> MKLSRISAINWNKIQDDKDLEVWNRLTSNFWLPEKVPLSNDIPAWQTLSAAEQQLTIRVFTGLTLLDTIQNIAGAPSLMADAITPHEEAVLSNISFMEAVHARSYSSIFSTLCQTKEVDAAYAWSEENPPLQRKAQIILAHYVSDEPLKKKIASVFLESFLFYSGFWLPMYFSSRGKLTNTADLIRLIIRDEAVHGYYIGYKYQIALQKLSAI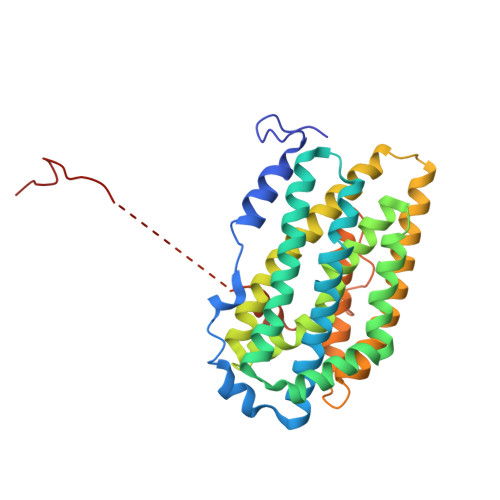EREELKLFALDLLMELYDNEIRYTEALYAETGWVNDVKAFLCYNANKALMNLGYEALFPPEMADVNPAILAALSPNADENHDFFSGSGSSYVMGKTVETEDEDWNF> SVQNNKFDEFGEWLLKESNGSKDDLPSDVEIYKRIVELEIADTPETLQVLGQVLFDDDIINQIEPHVGLLT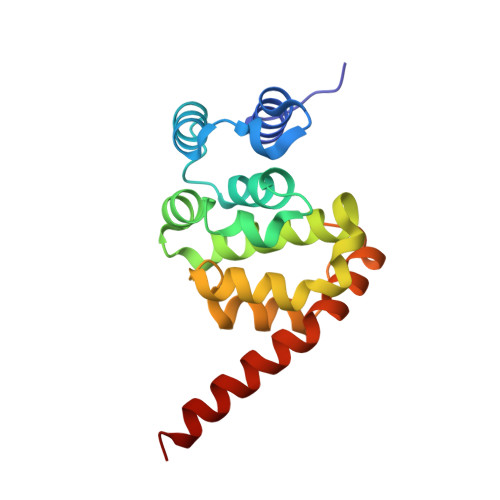KLINGDEEFEKALLGGLERFFGLEKPNLIPQIPKILHGFYDRDLISEEVLIKWGSKVSKKYVPKDVSKKVRKAAKPFVKWLQEAEEEEEEESD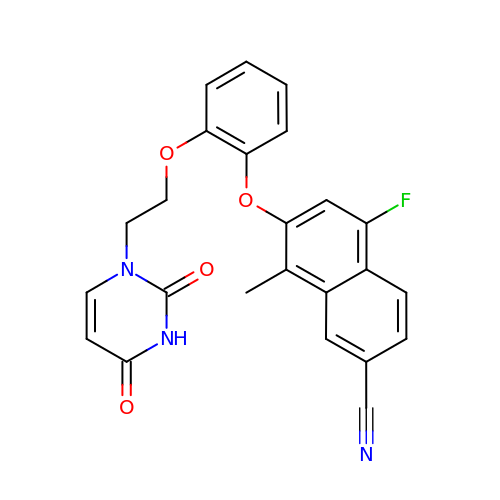7-{2-[2-(2,4-dioxo-3,4-dihydropyrimidin-1(2H)-yl)ethoxy]phenoxy}-5-fluoro-8-methylnaphthalene-2-carbonitrile | C24 H18 F N3 O4 | OIPOKGOOHCBAPR-UHFFFAOYSA-N> AGAGGGELFATHCAGCHPQGGNTVIPEKTLA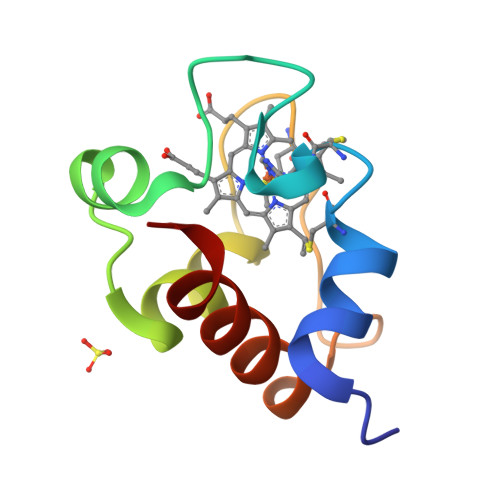RARREANGIRTVRDVAAYIRNPGPGMPAFGEAMIPPADALKIGEYVVASFP> MNKVWDRIVGSDSADAQSVLKERCSSPKDVTDLLHVIQNWTSEIHNNGEETRCWKCVPMLAGYVKDWGQLEFLCRRILLRSSIQEIRPLLLVTMKSLMSNHSDNTEQKCGNILQQLLIEAEEDSGNVSLRLLVDAMSLVFPICLGVCRDMFLSTD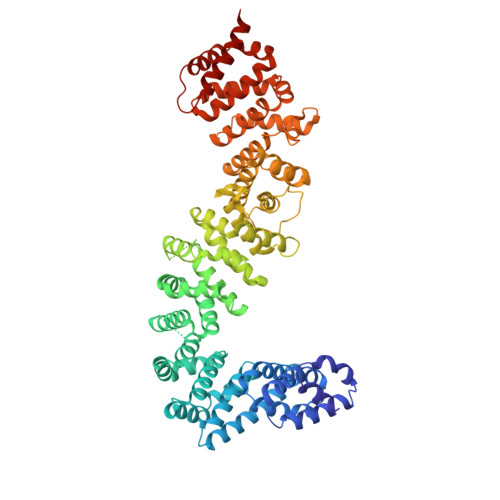FQDILTRNLNSSADDEHLVNGALRLLAVSCIDEAVRRFIAEHYLKTLQQSFKVEKYKVLTALVLIKIWSFTKIEKETLNSCINLFIDSLSNGENIEINTEALAYLTLKPSVRVLLRGNGDVCLKIIELIKSQDTTPTDLYGLLIILANVSEHPSQNEDTVDKLKASLKTNQEKNDEPTLENVKDIEEFNRDYIIDLDLIGSLKSIKLSTSSYNQAIRIIYNVTRDKTQISECVKQGAGLMLLVFLAQKRNLSKDEWYLLSIRALSKTLIYVNPETAFSKYSPLSAAPFLFENLPLPNDNALSELQFTQLDTYEALLALTNLATINQGVDLGKIILSNAQYWDSIENLLLDSSVRIQRSTLELISNLMSNPMAISAKFFCFENPKSAQNFEILVKLLELHDIQSQRAVAAIFANIASTVPFICKELSEKRNLIETAIRVFKTQNTDTDLRIRLLVLLSSIFNANAHAVACVKNDEEFVKELQKYRNTPSQKDPLTPELSKEILSLINLEHHHHHH> MGSSHHHHHHSSGENLYFQGGTMYDFEYLNGLSYTELTNLIKNIKWNQINGLFNYSTGSQKFFGDKNRVQAIINALQESGRTYTANDMKGIETFTEVLRAGFYLGYYNDGLSYLNDRNFQDKCIPAMIAIQKNPNFKLGTAVQDEVITSLGKLIGNASANAEVVNNCVPVLKQFRENLNQYAPDYVKGTAVNELIKGIEFDFSGAAYEKDVKTMPWYGKIDPFINELKALGLYGNITSATEWASDVGIYYLSKFGLYSTNRNDIVQSLEKAVDMYKYGKIAFVAMERITWDYDGIGSNGKKVDHDKFLDDAEKHYLPKTYTFDNGTFIIRAGDKVSEEKIKRLYWASREVKSQFHRVVGNDKALEVGNADDVLTMKIFNSPEEYKFNTNINGVSTDNGGLYIEPRGTFYTYERTPQQSIFSLEELFRHEYTHYLQARYLVDGLWGQGPFYEKNRLTWFDEGTAEFFAGSTRTSGVLPRKLILGYLAKDKVDHRYSLKKTLNSGYDDSDWMFYNYGFAVAHYLYEKDMPTFIKMNKAILNTDVKSYDEIIKKLSDDANKNTEYQNHIQELVDKYQGAGIPLVSDDYLKDHGYKKASEVYSEISKAASLTNTSVTAEKSQYFNTFTLRG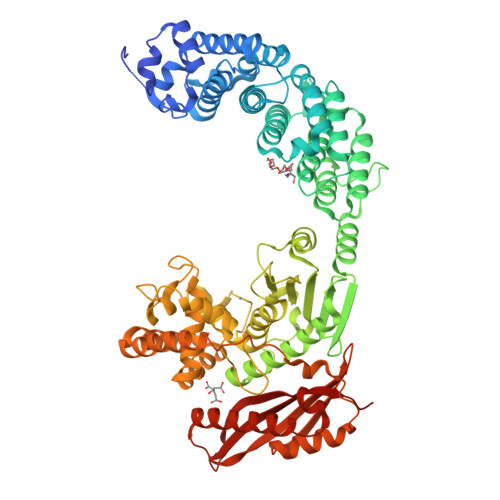TYTGETSKGEFKDWDEMSKKLDGTLESLAKNSWSGYKTLTAYFTNYRVTSDNKVQYDVVFHGVLTDNG>[2x]GTRKCELQGLWRNELGSNMTISALDVAGTFSGSYQTAVT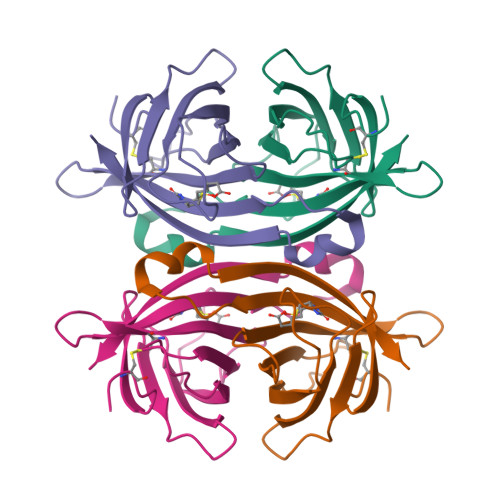ATNKQILVSPLKGAQQPPGTKGQQPTFGFTVQWQFADSTTVFVGQCFVDRRGKEMLEMAWLLREEVPSRKDTWKATRVGTNVFTRVK>GAMGSHLQAPTWYGEPSPAAHWAFGGKLVQITPDGKGVSITNPKISGLESNTTLSEALKTKDFKPLINQRLVKVIDDVNEEDWNMLEKLSMDGTEEFLKEALAFDNDESDAQDDANNEKEDDGEEFFQQIETNFQPEGDFSLSGNIEQTISKNLVSGNIKSAVKNSLENDLMMEAMVIALDSNNERLKESVKNAYFAKYGSKSSLSRILYSISKREVDDLVENLDVSQWKFISKAIQNLYPNDIAQRNEMMIKLGDRMKENGHRQDSLTLYLAAG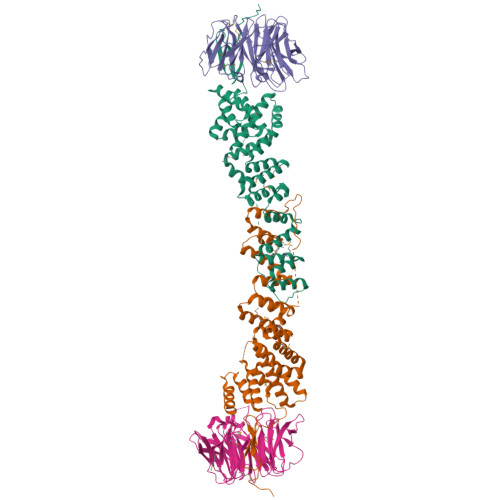SLDKVASIWLSEFPDLEDKLKKDNKTIYEAHSECMTEFIERFTVFSNFINGSSTINNEQLIAKFLEFINLTTSTGNFELATEFLNSLPSDNEEVKTEKARVLIASGKSLPAQNPATATTSKAKY[2x];>[2x]MVVIANAHNEMIHDAVMDYYGKRMATCSSDKTIKIFEVEGETHKLIDTLTGHEGPVWRVDWAHPKFGTILASCSYDGKVMIWKEENGRWSQIAVHAVHSASVNSVQWAPHEYGPMLLVASSDGKVSVVEFKENGTTSPIIIDAHAIGVNSASWAPATIEEDGEHNGTKESRKFVTGGADNLVKIWKYNSDAQTYVLESTLEGHSDWVRDVAWSPTVLLRSYMASVSQDRTCIIWTQDNEQGPWKKTLLKEEKFPDVLWRASWSLSGNVLALSGGDNKVTLWKENLEGKWEPAGEVHQ>MANVDEAILKRVKGWAPYVDAKLGFRNHWYPVMFSKEINEGEPKTLKLLGENLLVNRIDGKLYCLKDRCLHRGVQLSVKVECKTKSTITCWYHAWTYRWEDGVLCDILTNP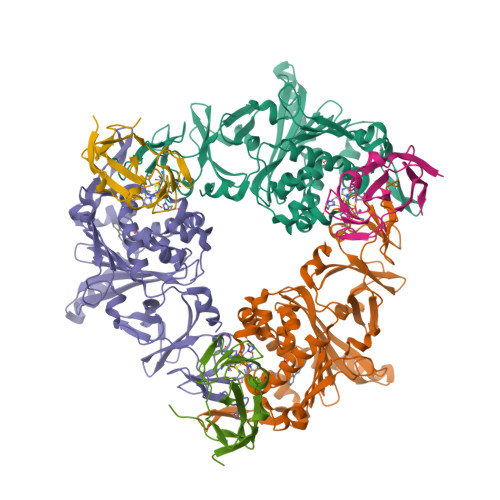TSAQIGRQKLKTYPVQEAKGCVFIYLGDGDPPPLARDTPPNFLDDDMEILGKNQIIKSNWRLAVENGFDPSHIYIHKDSILVKDNDLALPLGFAPGGDRKQQTRVVDDDVVGRKGVYDLIGEHGVPVFEGTIGGEVVREGAYGEKIVANDISIWLPGVLKVNPFPNPDMMQFEWYVPIDENTHYYFQTLGKPCANDEERKKYEQEFESKWKPMALEGFNNDDIWAREAMVDFYADDKGWVNEILFESDEAIVAWRKLASEHNQGIQTQAHVSGLEHHHHHH[3x];>MNQIWLKVCAASDMQPGTIRRVNRVGAAPLAVYRVGDQFYATEDTCTHGIASLSEGTLDGDVIECPFHGGAFNVCTGMPASSPCTVPLGVFEVEVKEGEVYVAGEKKLEHHHHHH[3x]(4~{S})-4-methyl-16,18-bis(oxidanyl)-3-azabicyclo[12.4.0]octadeca-1(18),12,14,16-tetraene-2,8-dione 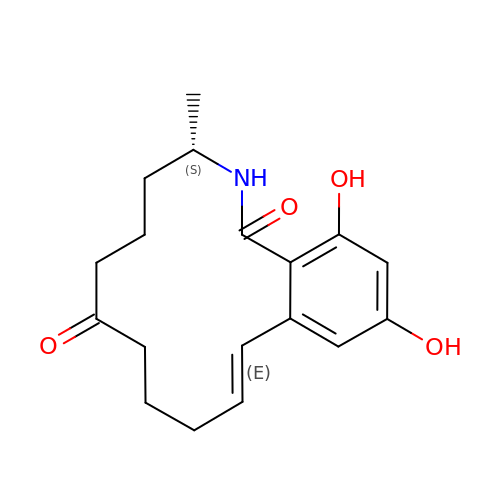| C18 H23 N O4 | MPCXTULDOJSSIB-QBODLPLBSA-N>[4x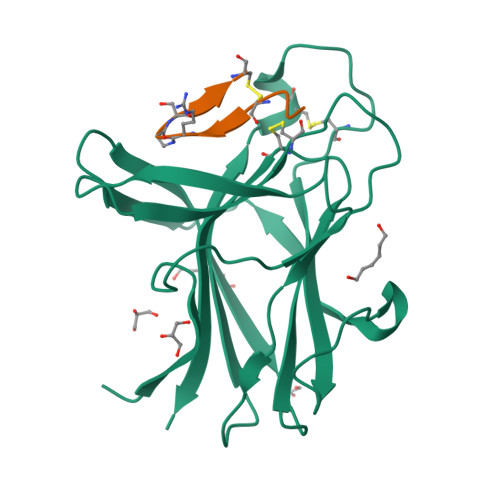]GPGNEVTLLDSRSVQGELGWIASPLEGGWEEVSIMDEKNTPIRTYQVCNVMEPSQNNWLRTDWITREGAQRVYIEIKFTLRDCNSLPGVMGTCKETFNLYYYESDNDKERFIRENQFVKIDTIAADESFTQVDIGDRIMKLNTEIRDVGPLSKKGFYLAFQDVGACIALVSVRVFYKKA;>APYCVYRXSWSCX[4x]>LQIFHYDEFSTASDKNRIRLQPLPPARGYIYDRNGVLLADNYPVFTATLSKADVENVDTVIEQLQPILELTQEDVDRFKSRIKTARKTERVAIKLNLTETNIAKFSEVKYKFPGVRIETQMTRYYPHGDLFAHVIGYVGRINDKELKSIDKDLYAGTNLIGKIGVEKSYEDLLHGTPGYESVEADAHSNILRHLGRKDPTRGNDLYLSLDYGLQVVASQQLAGRRGAIVAIDPRTGEILALVSSPSFNPNLFVTGINHKDYSSLRDNIDQPLYNRAVQGVYPPGSTIKPMEAMGGLHYGIVDWATAISDPGYFHLP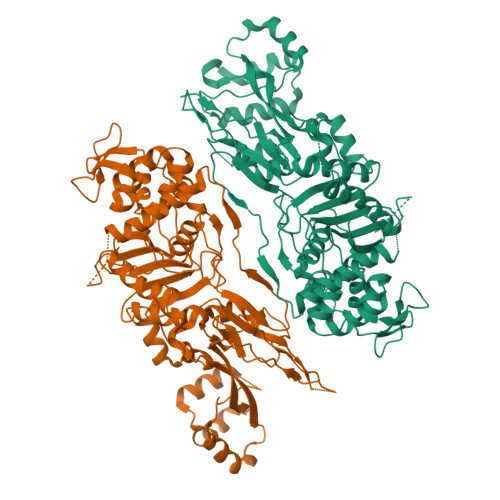GDSHKFRDWKKTGHGIVNMHKAIIMSCDTYFYILANQMGIDQMNQWMRQFGFGQKTGVDLPSESEGLYPNPEWKMRTRKSKWMKGETISVSIGQGAFTATPLQLAMATAITANHGSHVVPHVLRATHGAKPFTVRNAPDGKINFNGTDEDWVKMREAMIDVIQSGTGRGIRTPLYQIAGKTGTAQVKSIAQGKRYNEAALSERQLDHGLFVGFAPADKPEIAIAVIWENGRHGGSAAQLAKPVFDYWLLTRKKNPIRPANHQVNGGLMTAGIKPGELPSGNESASSTPATSAPTSAAASTPQATPTRPATNEVDE[2x]> ANVRLQHHHHHHHLEEFIADSKAELTLRNFYFDRDYKKDPYPYTAARDWAQGLIFKGQSGYTEGTVGFGVDVLAMAGFNLMGSRADDYARSGLLPVNTDNSRDDYYGKIGITGKAKFRKNELFVGDLVPQLPTIFSSPARLFPQTYRGIRFVSNEIPNLQLEGFYVDEVRQRDSIRYTDVGTDNINHRFNKAATTDSFYTLGGSYQLKDYRLRAYHAELKDIYQQQFLGFNGKQPLNDQLNFLSDVRFFNSEETG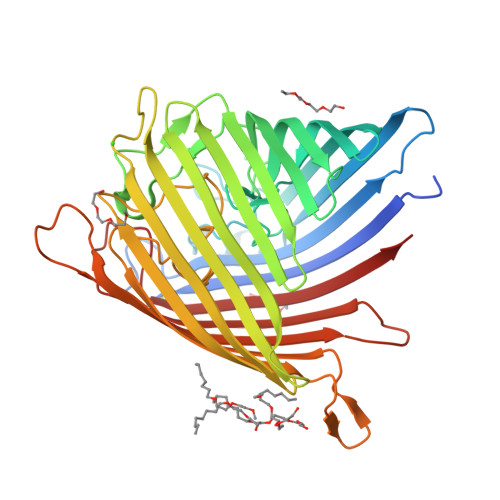SKKIGEVDNRHISGLFGLNYQNHTVSLGYMQSFGSTGLPFLSGTESPVVLDFMSSDYSNKDEKVYSIRYEYDFKNARIGDVSLNGLRFMTRYAKGEDIDLLQYGDQRFKEDSLEFDLGYKIPEGKLKGLGMRARFSHYRNDMPTNMTFHSANETRLNVDYTFKF> TVIEKRIVIDGDGDIDHDQALAQAIR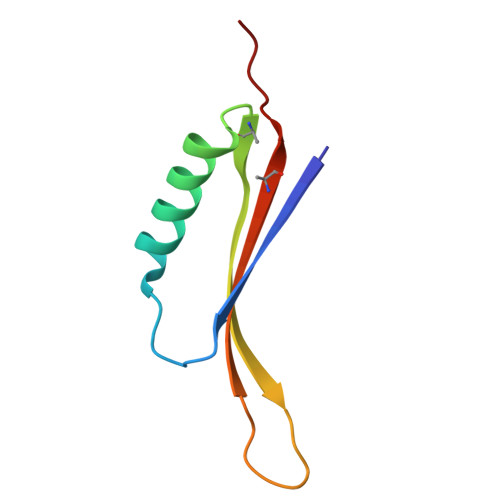EAREQHPDMSVTRVVVNKETELAEEGEDRTRQIINITMTKKLDVW>[2x]MNDLERLFNPSAIAVVGASKDPSKIGSQILRNLLSYGFKGKVYPINPTADELMGLKCYPKVSDVPDKVDVAVISVPSDKVLGVIDDCGKAGVKFAVVITSGFKEVGNEELEEELVRRAHSYGMRVLGPNIFGYLYAPARLNATFGPKDVLSGNVAFISQSGALGIALMGYTVVENIGISSIVSVGNKADLDDVDLLDFFDKDPNTGVIMIYLEGIAPGRGRMFIDVASRVSLRKPIIVIKAGRTEVGARAAASHTGSIAGSVAIYESAFKQSGILMAKSVEDAFDWTKALSWNPIPEGERLIVLTNGGGAGVQSTDTFADNGIYLSKPPESLIQEIKKFVPPFASFANPIDITGMAPDDW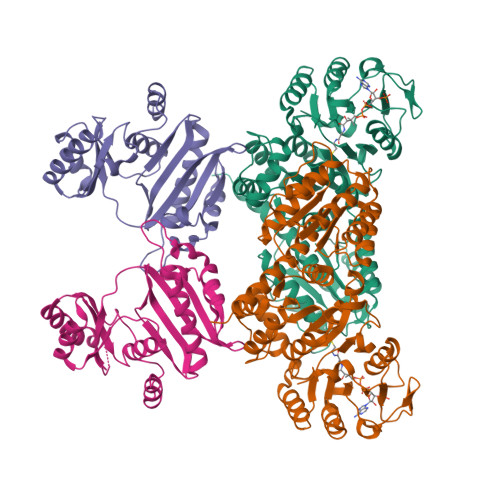YYMGTLAALKNPDVDALTVLYCQTAVTTPIGVAKGIVDAIKEAGNSKPVTVGMVGGPEVAEAVSFLNKQRIAAYPTPERASSAMSALYAYARARSYVMKSLAVR;>[2x]MSSRDLLLKAKENGRKSLLEHEAKYFISSYGIPVTNIRLAKSEEEAVNFSREIGFPVVLKIVSPQVVHKSDVGGVKVNLRSEEEVRKAYREIIENVKRNVPNAEIEGILVQEFAPPGVELIIGLLRDPQFGPTVMFGLGGVFVELFRDVSFRVAPLSEQDAESMIKEVKAYKLLTGFRGMEPVDIEAIKDALIRAGRIGVENEEIAEMDLNPVIAYPKGIKVVDARIILR>[2x]VKSKAKKTVDKHSDEYKIRRERNNIAVRKSRDKAKMRNLETQHKVLELTAENERL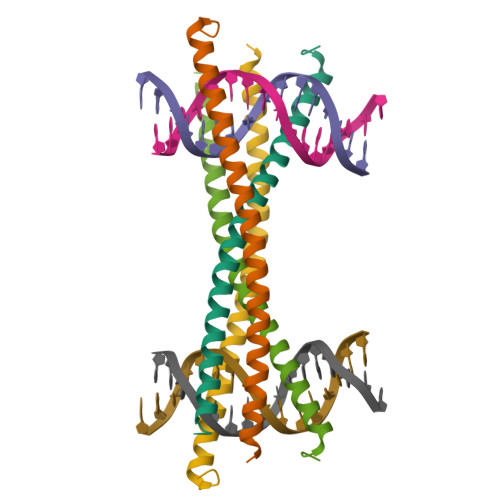QKKVEQLSRELSTLRNLFKQLPE>GRVRIEKMSSEVVDSNPYSRLMALKRMGIVSDYEKIRTFAVAIVGVGGVGSVTAEMLTRCGIGKLLLFDYDKVELANMNRLFFQPHQAGLSKVQAAEHTLRNINPDVLFEVHNYNITTVENFQHFMDRISNGGLEEGKPVDLVLSCVDNFEARMTINTACNELGQTWMESGVSENAVSGHIQLIIPGESACFACAPPLVVAANIDEKTLKREGVCAASLPTTMGVVAGILVQNVLKFLLNFGTVSFYLGYNAMQDFFPTMSMKPNPQCDDRNCRKQQEEYKKKVAALPKQEVIQEEE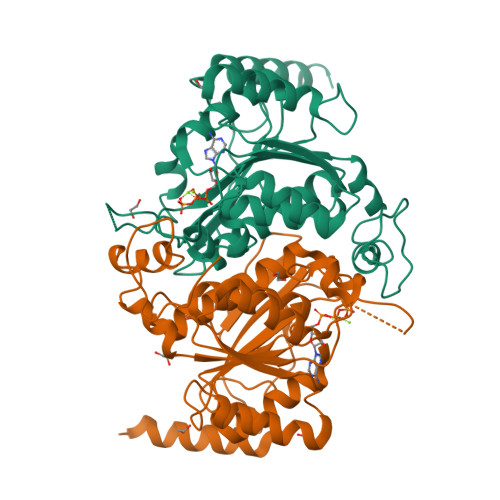EII[16x]>APQQINDIVHRTITPLIEQQKIPGMAVAVIYQGKPYYFTWGYADIAKKQPVTQQTLFELGSVSKTFTGVLGGDAIARGEIKLSDPTTKYWPELTAKQWNGITLLHLATYTAGGLPLQVPDEVKSSSDLLRFYQNWQPAWAPGTQRLYANSSIGLFGALAVKPSGLSFEQAMQTRVFQPLKLNHTWINVPPAEEKNYAWGYREGKAVHVSPGALDAEAYGVKSTIEDMARWVQSNLKPLDINEKTLQQGIQLAQSRYWQTGDMYQGLGWEMLDWPVNPDSIINGSDAKIALAARPVKAITPPTPA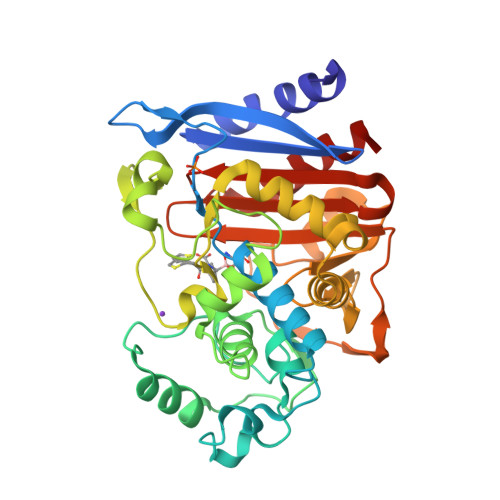VRASWVHKTGATGGFGSYVAFIPEKELGIVMLANKNYPNPARVDAAWQILNALQ[2x]> MRSVISEQSLASTKTQKLFNNLISKGQSKIPLLEGQLDEESLTKTWGAFGLYLSRQLRMGRGTNIPHFGTFTFSAPECNLTGVTNPIERDKQFRVPVFLVSKEFVLGQPIKTGIFIDKHIRPYNVQTSGSISVTKINFTEIAQYADQNKEAVKISFERIIRQLADQTRQKRVVDMEIPGIGVFQVRNNIAAVHFDEYLIQNIKGVPKRPLSERKQKGDMNLTADRLSMLENTSRIGADAEQYLKTKLGIDIDNISTKSRPLTAVRNASTSNLLQPNNKTLQRPATSTTLRQSAINLKQPELGPLEFGLKRLKFWIRQNCFNAQDAFLEMCNCALGRTRAQRVKVDYKQFFEAINKMELDLNEEQIQELFKQLDANKDGYINYTDWRNTIKDDNDHLQYIKDVIYKRQLHTDDVLKTMGLDREHPPINKYQLKDALKKLDLTLTDIKAIRVAQTLLGHEEYISMYDLARSFETIEEDDKIFDPSWFKDILYKIKQKIMALENPNEIRESFENYDEHNEGILDTANFKTCLMRSQLKLTVKEINRIVRYLPKVKVNNIDYYNFLKLVERVDINASAPDAVSDISEFAVKLGKFIKDKKFTIPSFLKTVRRFSFVLDSSNNQDYFVTLTQMSEFLHRNVFKGNDRLDIDFYVNELDIDCDGYIKENDVQSFLNRYTYFDQ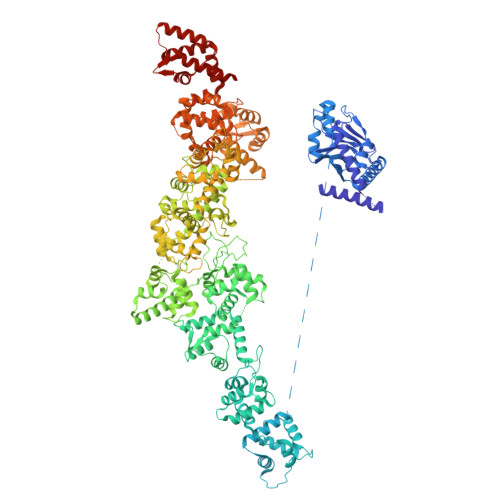TQYTPLSMTRSLTLKSLDPRTVSMNTKTLYPFKALSEAKVDTILRDLRKKMELKKMKAAELFSTLDADQDGFLTINEFSENIRKIIELSQPAIDGFFAYMDKLHTGMVDLSSFLKVMRKSIVTKDQPIKEDNFDWENEMVFRIRQWFKKEGITVEDSFRAIDQNFKREINVDDLEIFLKDCLKVKSEELNKAKLDRLFKLIDQYKRGKVNFVDWKRFIMEDFGYGMNQTIMGGKKIDNISSFDWKINARQQLGLVLTRRFSTLSHSFDVISGYRKKLLFSHFKKWVQDTDALRGFDLTESLMQELFSDLDSHNKGYLSESDWEIAFGGFDWEHQMHEEIKEYVKQNFKSIEKAFEFFCQGNQNKIIEQADFNKAINSILPKRFIDSDLKDLWVYVSSGQPQVDFHRFKIAFQKYIPHYERTIEYDQENMRPKTAGPLSSLSKSTSWNNIYGASQLNGNSQNPFGTSSIVDGNEDDVFEEKLLSKIRRLLRPTIKSVKKVLEQLDVNNIGYITNLEFRNAIKTLNLGLAQNEVDLLLNICEIDGRVNIKQFLKFIDFSESDKKIVQRSILKLREITNQVYTFLLSPKDAFRMFDVDSNGYLDFDQFSQFIGKLSQLSGHDMLPYSIIKDLFEYIDSKKDGVIDQAEWMDIFNKFEYVPQASINKQPLSKATVYNLQKRPQTSFNKSTLNELPHNKFNLEYISSNYPLTVKNEKIHQISDKEKYGTMNKFFDEVERQPESKPVQDNHFNQILGEWGKTKEFDKIIISIGKNRRFLLDMFGSLQQRNIPITFERAKAIIGQMLRNSGQSLKEESWPIILKFAERNGLIDYKFLLEVYKERIKRIDSHPIMSRNRSLQKFTS Tilapia Lake Virus (TiLV), a recently discovered pathogen of tilapia fish, belongs to the Amnoonviridae family from the Articulavirales order. Here we show that segments 1–3 encode respectively the PB1, PB2 and PA-like subunits of an active heterotrimeric polymerase that maintains all domains found in the distantly related influenza polymerase, despite an unprecedented overall size reduction of 40%. Multiple high-resolution cryo-EM structures of TiLV polymerase in pre-initiation, initiation and active elongation states, show how it binds the vRNA and cRNA promoters and performs RNA synthesis, with both transcriptase and replicase configurations being characterised. Recombinant TiLV polymerase specifically binds the conserved 5′ and 3′ genome and anti-genome ends, with mode A and mode B promoter structures similar to other segmented negative strand RNA viruses.

To structurally characterize the early elongation state, TiLV polymerase was incubated with the 40-mer vRNA loop, the capped 13-mer primer ending in …CC-3′, ATP, UTP, Mg2+ and CpNHpp. This leads to elongation of the primer by eight nucleotides to become a 21-mer, before stalling at nucleotide G11 of the template (Fig. 7b, lane 5). Two distinct elongation structures of TiLV polymerase were determined from the cryo-EM data at respectively 2.96 and 2.42 Å resolution. Both show the full-length TiLV polymerase with CpNHpp bound at the +1 position and a product-template duplex filling the active site cavity. Unusually, the product-template duplex comprises 11 base pairs (+1 to −10) where generally for viral polymerases a maximum of 10 base pairs is observed. This likely arises from the PB2 lid domain not yet having managed to completely clamp down and enforce strand separation compared to the late elongation structure presented below. The CpNHpp is bound in a non-catalytic configuration with only one magnesium ion. Although a capped primer was used to initiate the elongation reaction, the cap itself is not observed and the putative cap-binding site remains autoinhibited by PB2/R217. The higher resolution structure with the additionally bound 3′ ends mimics a later elongation state in which the outgoing template would have translocated into the 3′ end secondary site.

> MDSRFAQLTGVFCDDFTYSEGSRRFLSSYSTVERRPGVPVEGDCYDCLKNKWIAFELEGQPRKFPKATVRCILNNDATYVCSEQEYQQICKVQFKDYLEIDGVVKVGHKASYDAELRERLLELPHPKSGPKPRIEWVAPPRLADISKETAELKRQYGFFECSKFLACGEECGLDQEARELILNEYARDREFEFRNGGWIQRYTVASHKPATQKILPLPASAPLARELLMLIARSTTQAGKVLHSDNTSILAVPVMRDSGKHSKRRPTASTHHLVVGLSKPGCEHDFEFDGYRAAVHVMHLDPKQSANIGEQDFVSTREIYKLDMLELPPISRKGDLDRASGLETRWDVILLLECLDSTRVSQAVAQHFNRHRLALSVCKDEFRKGYQLASEIRGTIPLSSLYYSLCAVRLRMTVHPFAR;> MWAFQEGVCKGNLLSGPTSMKAPDSAARESIDRASEIMTGKSYNAVHTGDLSKLPNQGESPLRIVDSDLYSERSCCWVIEKEGRVVCKSTTLTRGMTSLLNTTKCSSPSELICKVLTVESLSEKIGDTSVEELLSHGRYFKCALRDQERGKPKSRAIFLSHPFFRLLSSVVETHARSVLSKVSAVYTATASAEQRAMMAAQVVESRKHVLNGDCTKYNEAIDADTLLKVWDAIGMGSIGVMLAYMVRRKCVLIKDTLVECPGGMLMGMFNATATLALQGTTDRFLSFSDDFITSFNSPAELREIEDLLFASCHNLSLKKSYISVASLEINSCTLTRDGDLATGLGCTAGVPFRGPLVTLKQTAAMLSGAVDSGVMPFHSAERLFQIKQQECAYRYNNPTYTTRNEDFLPTCLGGKTVISFQSLLTWDCHPFWYQVHPDGPDTIDQKVLSVLASKTRRRRTRLEALSDLDPLVPHRLLVSESDVSKIRAARQAHLKSLGLEQPTNFNYAIYKAVQPTAGC;> MSQFGKSFKGRTEVTITEYRSHTVKDVHRSLLTADKSLRKSFCFRNALNQFLDKDLPLLPIRPKLESRVAVKKSKLRSQLSFRPGLTQEEAIDLYNKGYDGDSVSGALQDRVVNEPVAYSSADNDKFHRGLAALGYTLADRAFDTCESGFVRAIPTTPCGFICCGPGSFKDSLGFVIKIGEFWHMYDGFQHFVAVEDAKFLASKSPSFWLAKRLAKRLNLVPKEDPSVAAAECPCKKVWEASFARAPTALDPFGGRAFCDQGWVYHRDVGYATANHISQETLFQQALSVRNLGPQGSANVSGSIHTALDRLRAAYSRGTPASRSILQGLANLITPVGENFECDLDKRKLNIKALRSPERYITIEGLVVNLDDVVRGFYLDKAKVTVLSRSKWMGYEDLPQKPPNGTFYCRKRKAMLLISCSPGTYAKKRKVAVQEDRFKDMRVENFREVAENMDLNQGSGSENLYFQGHHHHHHHHHH pmcThe enzyme 2′-deoxynucleoside 5′-phosphate N-hydrolase 1 (DNPH1) (EC 3.2.2.-) is responsible for catabolizing toxic 5-hydroxymethyl-2′-deoxyuridine 5′-monophosphate (5hmdUMP), a noncanonical 2′-deoxynucleotide that, if incorporated into DNA, must be excised via DNA repair pathways. DNPH1 catalyzes the hydrolysis of the N-ribosidic bond of 2′-deoxynucleoside 5′-monophosphates to produce 2-deoxyribose 5-phosphate and the corresponding nucleobase.5HsDNPH1 also accepts canonical 2′-deoxynucleoside 5′-monophosphates as substrates, albeit with very low reaction rates. The dimeric form is common for DNPH1 and is essential for catalysis. The overall fold is similar to previously reported inhibitor-bound structures of HsDNPH1 and rat DNPH1,6−8 with a five-stranded parallel β-sheet core surrounded by five α-helices.

We solved the crystal structure of unliganded human DNPH1 and took advantage of the slow reactivity of 2′-deoxyuridine 5′-monophosphate (dUMP) as a substrate to obtain a crystal structure of the DNPH1:dUMP Michaelis complex. To investigate the structural basis for catalysis of N-ribosidic bond cleavage, the structures of unbound HsDNPH1Trunc and dUMP-bound complex were solved with data to 1.7 and 1.42 Å resolution, respectively. Omit (Fobs–Fcalc) maps showed electron density for dUMP but only in half of the binding sites of the dimer. The 5′-PO42– group of dUMP makes polar contacts with the main chain −NH of Ile29, Arg30, Gly31, and Gly100, the Ser98 −OH of one subunit, and the Ser128 −OH of the adjacent subunit. The dUMP 3′-OH donates an H-bond to one of the O atoms of Glu104 −COO– and accepts an H-bond from Gly27 −NH. The other O atom of Glu104 −COO– is locked in an apparent LBHB with the Tyr24 −OH. The uracil moiety of dUMP makes nonpolar contact with Ile76 of one subunit, and its 2-CO group makes a polar interaction with the −OH of Ser128 of the adjacent subunit. Glu104 −COO– sits underneath the 2′-deoxyribose moiety of dUMP, 3.8 Å away from the dUMP C1′, a position suitable for nucleophilic attack on the anomeric carbon of the substrate. The main change reflected in the active site upon dUMP binding is the stabilization of the Ile29–Glu34 loop via polar interactions with the 5′-PO42– group, with the side chain of Arg30 closing as a lid over the substrate. An intriguing hypothesis for this observation invokes the enzyme harnessing the binding energy for the 5′-PO42– group to drive a conformational change that traps the substrate in a caged Michaelis complex conducive to catalysis.

>[2x]GMRPALYFCGSIRGGREDRTLYERIVSRLRRFGTVLTEHVAAAELGARGEEAAGGDRLIHEQDLEWLQQADVVVAEVTQPSLGVGYELGRAVAFNKRILCLFRPQSGRVLSAMIRGAADGSRFQVWDYEEGEVEALLDRYFEADP PNGM-1 is derived from a metagenomic library from deep-sea sediments that predate the antibiotic era. PNGM-1 has both MBL and tRNase Z activities and is considered to be the evolutionary origin of B3 MBLs. The wild-type of PNGM-1 has two MBSs in its substrate-binding pocket, and each is occupied by a zinc ion. The zinc ion in the first MBS (Zn1) is coordinated by the residues His91, His93, His188, and Asp210; the zinc ion in the second MBS (Zn2), by Asp95, His96, His279, and Asp210.

We determined the crystal structures of five PNGM-1 variants: H91A, H93A, H96A, H257A, and H279A. His257 is not directly involved in metal coordination but plays a role in the tRNase Z activity of PNGM-1. As His257 is distant from the MBSs and not involved in metal binding, the Zn1 and Zn2 in the H257A variant are occupied by metal ions. In the structures of all PNGM-1 variants, except in that of H96A, the electron density corresponding to the catalytic water remains despite the complete or partial loss of a zinc ion.

>AGGKVTSSTGIAPKRYVYYPGSEELGPDEIRVIACGTGMPTARRAQAAAAWVVELGNGDKFIVDIGSGSMANIQSLMIPANYLTKIFLTHLHTDHWGDLVSMWAGGWTAGRTDPLEVWGPSGSREDMGTKYAVEHMLKAYNWDYMTRAVTINPRPGDINVHEFDYRALNEVVYQENGVTFRSWPCIHAGDGPVSFALEWNGYKVVFGGDTAPNIWYPEYAKGADLAIHECWMTSDQMMTKYNQPAQLALRINLDFATSAQSFGQIMNMVQPRHAVAYHFFNDDDTRYDIYTGVRENYAGPLSMATDMMVWNITRDAVTERMAVSPDHAWDVAGPSEDLAPDRNRASEYTQYILDGRLNVDEANAHWKQEFMG[4x]> PTSENPKIGPI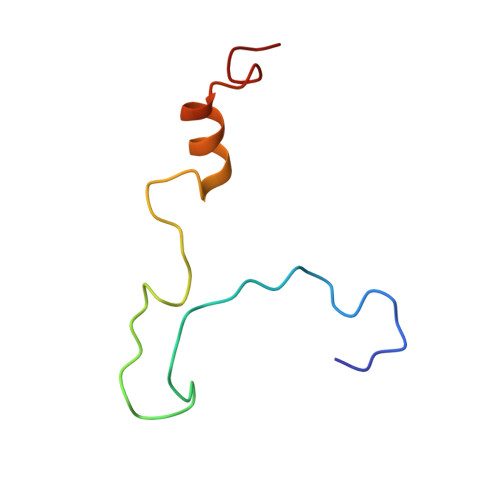SEVASGVKTAANGIERIPVLGEIAKPVTAAVKWFADIVGGVAAIFGW>[2x]SRLNRESVI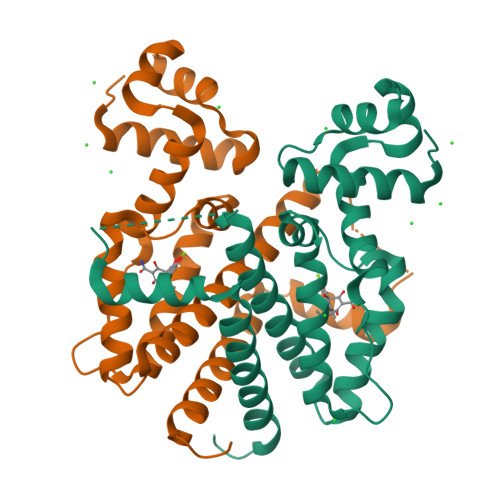DAALELLNETGIDGLTTRKLAQKLGIEQPTLYWHVKNKRALLDALAVEILARHHDYSLPAAGESWQSFLRNNAMSFRRALLRYRDGAKVHLGARPDEKQYDTVETQLRFMTENGFSLRDGLYAISAVSHFTLGAVLEQQEHTAALTDRPAAPDENLPPLLREALQIMDSDDGEQAFLHGLESLIRGFEVQLTALLQIV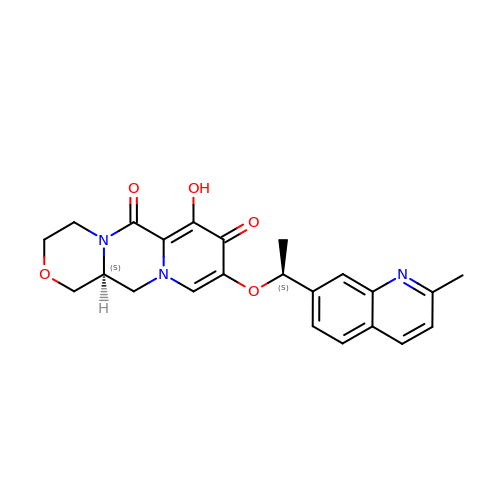(3~{S})-13-[(1~{S})-1-(2-methylquinolin-7-yl)ethoxy]-11-oxidanyl-5-oxa-1,8-diazatricyclo[8.4.0.0^{3,8}]tetradeca-10,13-diene-9,12-dione | C23 H23 N3 O5 | DPINYONVCPWSBW-YOEHRIQHSA-N>MNKTDLINAVAEQADLTKKEAGSAVD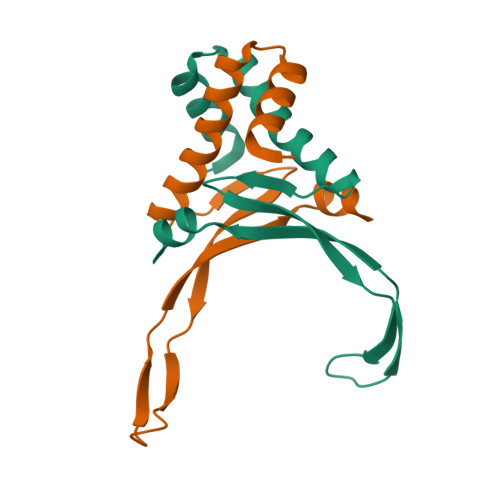AVFESIQNSLAKGEKVQLIGFGNFEVRERAARKGRNPQTGKEIDIPASKVPAFKAGKALKDAVKLEHHHHHH[4x]>MSLLNVPAGKDLPEDIYVVIEIPANADPIKYEIDKESGALFVDRFMSTAMFYPCNYGYINHTLSLDGDPVD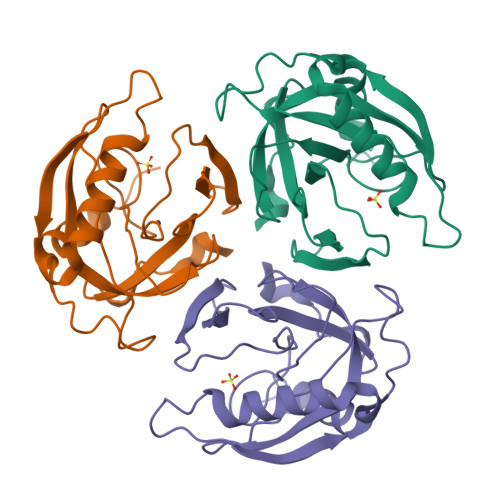VLVPTPYPLQPGSVIRCRPVGVLKMTDEAGEDAKLVAVPHSKLSKEYDHIKDVNDLPELLKAQIAHFFEHYKDLEKGKWVKVEGWENAEAAKAEIVASFERAKNK[3x]> MADVAGTSNRDFRGYILSVQAEEQKNYNNSLNGEVSVWVYAYYSDGSVLVINKNSQYKVGISETFKALKEYREGQHNDSYDEYEVNQSIYYPNGGDARKFHSNAKPRAIQIIFSPSVNVRTIKMAKGNAVSVPDEYLQRSHPWEATGI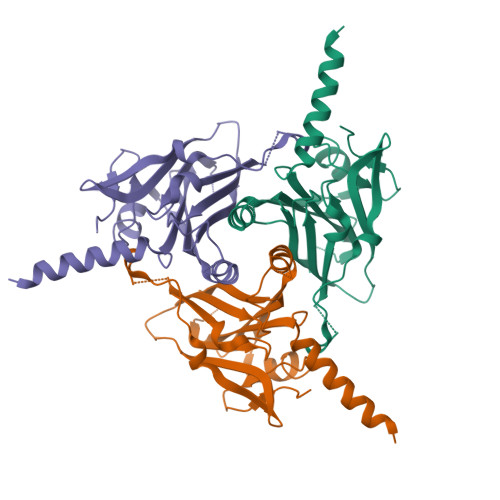KYQKIKRDGEIVGYSHYFELPHEYNSISLAVSGVHKNPSSYNVGSAHNVMDVFQSCDLALRFCNRYWAELELVNHYISPNAYPYLDINNHSYGVALSNRQ>[2x]MSWQAYVDTSLLGTGKIDRAAIV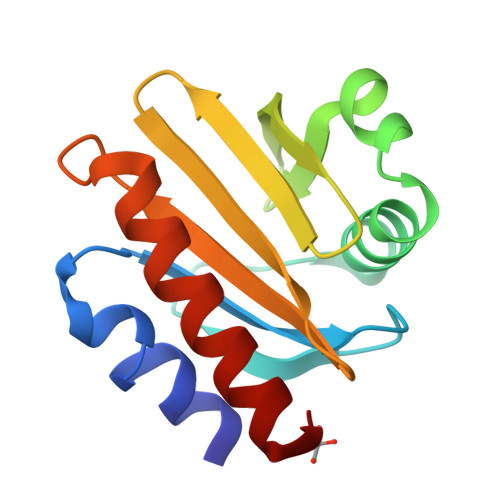SRAGDSVWAASAGFNLSPQEIQGLAAGFQDPPSMFGTGIILAGQKYITIRAEGRSIYGKLQKEGIICVATKLCILVSHYPETTLPGEAAKITEALADYLVGVGY> MRRRVVLCCQDVGSLLSSKHSVHSGIGYHERVFSRNLLYRRYPVVTVLPKAGFTVLDTKRWIASSGPPVTGSPLSPVTNPSLNVGTGGGEAVAMEGPLPVSYSPGSGVNGSLPVTSTAITAHCDVLSECVAKADELAVQLKAQNALSASAEILTQEGMEEFVEELKTSATNEMTALVKQMQTTPLLQRAGMHELRRTLYYTTSLKERDWLEEKQYTAAMRMLTVEVLRRDGDGVLSADDVLYVTTHVVTANFYNRHLWNRMEKSLLKFSNYENIDMSSVKAFSTRLFKTRRGCAKETLDIRRKVLLAMSRRVGVLANDFDLPSLLGVLQCYTVHDLTPFHLEPLAIRATNHVGDFTPHECATLAHVLRKWRTMRLEVCERLVERICTSDQLTHHMANAAMIAIRTCFNQVSDGGRNAMNAEPTRQKLRAMGEQIGCRLDEVEYPALPVILSILDVVVTLKIYVPKKCLQVIFSQANDMVAIVMEQKDDLVDPKTGKRVRPITAEEGRQLQALLSHYGNDLAPELSQRMKEAFREGVLPDEASL;> MRSGRKLGCFTNRLRLPFFSPCSQITALTASHRCKSYVLKFLRGQLPEDLKDVNGALGCLYGTLPDVDEFGQFVISPDVVNSFHQFGYVKMPIPVLDHQQIDKLADEVNELANNVEHHPKTERLYATSLADLTGGPLFFCQGQWRAAWGMHDLIYLPTITVAASQILNNSLVRLWYDEVFMKAARTGPCVPWQQNYARWQHTKPVNHVTVMIALDTMNKDRGAPCLVPGSHRWREGGLLPPVSYDPTKDEAHQLNTIWEIINEEEGEMLMDTPPVTVDLRRGEALLIHPLTLFATHGNRSLDAVRCCFIHYMGEKTYAVQNGPLLPHTTKFQADAMIQGPFYPVVFDPAMTEELTMLPTAPSEEEA;> MLRHTSRNNALHAFVRSPHYRTIPSAGPNGIVVNRDMLVHQFRDFYKTLQHCSLVDKVHLMSERPSVEALRVADQMVSIGATFLEMPLTGMEHRATEFMESMRYVRGAGGPSTLASYLQDTENCRCNSGDVVCLPNGIAVGHGPRTNAVAHTTLKQLFEVKDDQFSFDVFTLEQEGDAPPLGDYFGFAGSNVLLTWKDEHGLLAVDQYQQKQPHTEMNVVYLEPGCHFLSFYGVDHTIDVLVQKGYERSMDSIAAAGLNPIPVQWSEMDKLGISMRAAVLPLKFFKANVGGMLSRNKSRGARWQTHQLQK;> MRSALRRCILRHQGCLRMKQSLSAFPTVVTGMTRHQGNSLIGTTHGAELSLAGDPQSVSHLSARNIATEALQMKKLHQERGGNPMLAQQARRVLFATSIAGQNLDARSVALLLNTAVYFGMESDAKLVRECIDYCLKNDKLITVDVLPIVVTACATLKSRDAREVIEMQAQKAARNAKFLDAKDVTNIISAFSKTGINHEKLFAFLSRRVQTLARVGEFEAAHLVILANAFSRLRYRDKFLFGAIARRAMSLRERVTVNELVPLIVAFSKIGLKDPKLSKRFATKAMEYVDQMNAEQVASMFMAFAYFGIRYDQLFGVLTNRAVELIDEFNAQYISTTLNAFQRIGINNPELFDNLAERALAVVQDHDARDISKTVTALAHFGLKDEELFKRLASHAASIADQFDAMGLVNTAHAFARTNFLQQDMAVALSERSVYVCRLLDAGETRRLLWALAKFQVRDPKILTPVFNRCLALHYDFFADPTGSEEIEEIFDFYGPNFCPPLYQLYISRGSTPQA;> MRSSRGILFLSGAFAIRGMSAYHSYQRLDTVSHTSKVYSLQMQRQTVHFTPITRLGVEATANPTTATNATGQTGDGDGATALDVAMRVNKLKRLHQTGGGPSGKKQVELDAWRDLNNLTEAQINSAEGKAVSLLLNSWAYFAKYWEKGAEGPSASLSEVTPSNDSSSAGEHGTQ;> MLNVLSSTASAALATVVVARPSALHLIFERCKLNLVEFTAQDVYQICTTAYNMDTLGMLQDPDFMRGLHDAFRRSDQTVISPFQANLIADTFRKVGINSMPKEVSVPEEDAISPESLILVLRNMNITKQRDERKINEVLK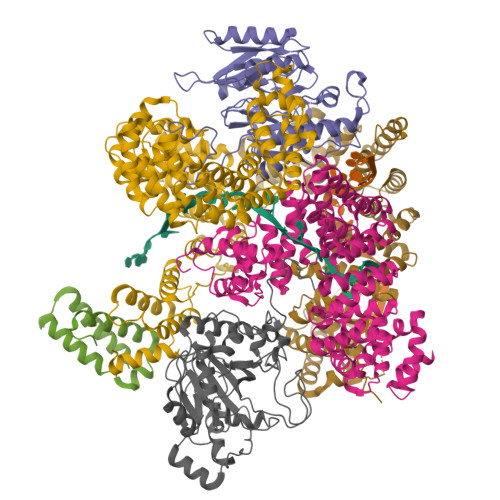LMFPILDEFSPTQLSLTVTELARLKSTNADFVGKLAKRIMEYNDDLSALDISSAAVSLAYCPGISHNILYRMMQIVEERMGEFQPEDYINVLHALNTLGPKFVNTFRKIVECGLQHVENMDAVTLTNYMVCFSTMDYKQREHIDIYADALVEVATDLSEKDLVMAFIALQRLRLLSDTMFGTMASCVIRYAAKMDPRNIAPIMDICSTVPHASDHLMKVLMDRAVECTRILTANQLGDILDILGLYPPAREHPLVQLFGKQARLRLDLMGPDALANATRGLANLGYADPEYYAQAAETGFRYGFKDWTLLEPMLMGLSITGQCPPTMVRVLGSHIAPMARSMSLMEIERANRYLRRLGCEDDFVYKAMASRVLQFVKEVTPEMPEDLQVLLQRGAVEPGAAPGVM>[9x]MAYPYSDMPFGVELDTSTLGSFGLGGPQTQLQMQMPAVDVNAAASGSGGFMAGFSNIFSRDSMFGGVAPSGAQTGGWVLPALGIGQAVFGAIGANRQQRA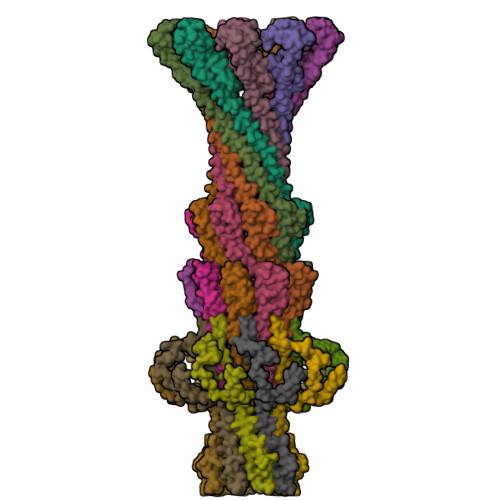ARDQLAESRRQFDMNYGAQRQSINTNLEDRQRARVASNPTAYESVDSYMERNRIR;>[9x]MAQEITWRNIGATVSPGSASSMSAGTTGVQQALGALGDIISRQQEMNVNNAKLQREANTQSYLDQVAASTLEQLSNADYRSGLEAQRDAMGMNLDRAATRDAITKQISAQQNQAAATQKFDDMQAEVGQRGIVDQLRTLSAEGRAGEVNQILAEQQLINEGEIRKELTGVQDAIQNRQYRAAGEQRAQAAANRAAEAHSLSMAAGRENLAFTREQRDELRRDRDEAKLVSGTIATTFQDYDESRQAQSEIMRIVGKEVGMPTDDQGMPDMSRASQDQLDAFSNALNEAGVQANTSPTERRNAVLKSLVDAGVSSKGIAQAKQEMELRESLEGLAPQDRTKVEATIGAVNAELDTLQRTATEDYEREVARNPFVEPDKDPLGSVNKIVDKAVKSGFGWEGDRQDLNNMLVDFATNGIKLPDGRTAVVPSKLLEQAFNTTNTWLFKNAGDVEKRIIELMTTDGMTQMREDAPTIRENFLKTVSDIANQKRSNAVKVTRSAEREKGVTMDPTDDLTFALRGRKR(3S)-3-(3-fluorophenoxy)-1-methylpyrrolidin-2-one 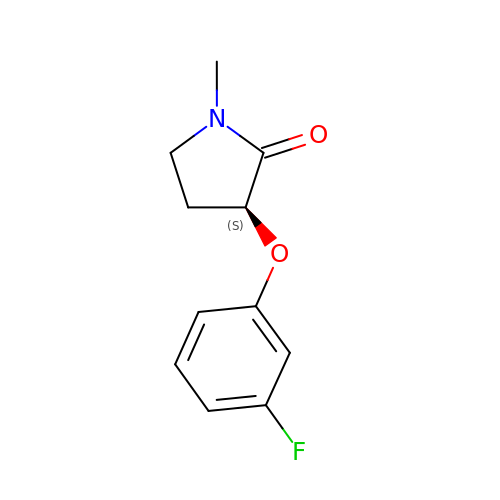| C11 H12 F N O2 | JWLJWMCLUCDWSD-UHFFFAOYSA-N>MGAERDESGAGAAVLVPLLGFGSNRPAGPAEKMAVAGSGWSLARVAEALGSSEQALRLIVSILMGYPFALFQRYFLFQKETYLIHLYNVFTGLSIAYFNFGMQFFHSLLCVLIQFLILRLMGRTVTAVFTTFVFQMTYLMAGYYFTATEHYDIKWTMPHCVLTLKLIGLAIDYYDGGKDPELLTPEQRRFAVRGVPTLLEVSGFSYFYGAFMVGPQFSMTDYQKLAKGEMTDVPGQRPNSFVPALKRLSLGLLFLVTYTLSSPYISEEYLISDDYMEKPFWFRCGYILVWGKIILYKYVTCWL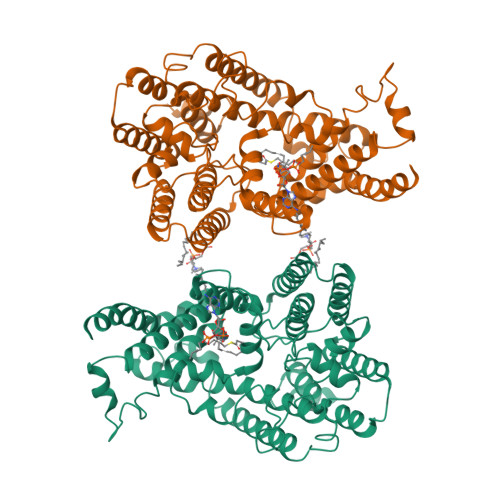VTEGVCILVGLGYNGNDQNGKPVWDACANMKVWLYETTPLFTGTIASFNINTNAWVARYVFKRLKFLGNKLLSQALALFFLAIWHGLHSGYLVCFQMELLIVIVERQVINLVRDSPTLSTLASITALQPIFYVLQQTNHWMFMGYSLVPFCLFTWDKWMKVYKSIYFLGHVLFFTLLLVLPYIRKLLVPRKEKLKKAE[2x]>[45x]ATLRSFVLVDNGGTGNVTVVPVSNANGVAEWLSNNSRSQAYRVTASYRASGADKRKYTIKLEVPKIVTQVVNGVELPVSAWKAYAS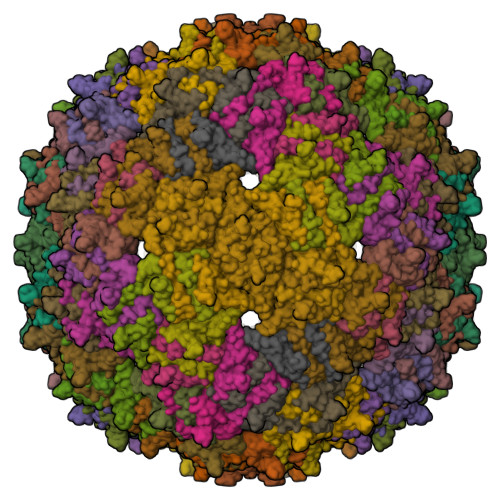IDLTIPIFAATDDVTVISKSLAGLFKVGNPIAEAISSQSGFYA>[3x]KETAAAKFERQHMDSSTS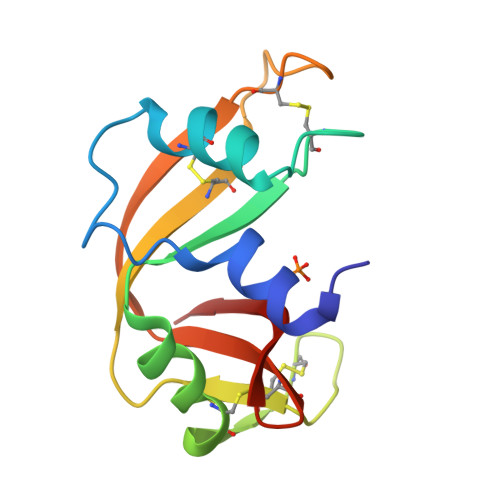AASSSNYCNQMMKSRNLTKDRCKPVNTFVHESLADVQAVCSQKNVACKNGQTNCYQSYSTMSITDCRETGSSKYPNCAYKTTQANKHIIVACENQAPVHFDASV>[5x]MNEAVKTLDGWFCLHDFRSIDWAAWRELNPGNQELMLNELSHFLSDMEITKNIGEGEHTIYSILGQKADLVFFTLRDSLEALNEVENRFNKLAIADYLLPTYSYISVVELSNYLASHMAGGDDPYQNKGVRARLYPALPPKKHICFYPMSKKRDG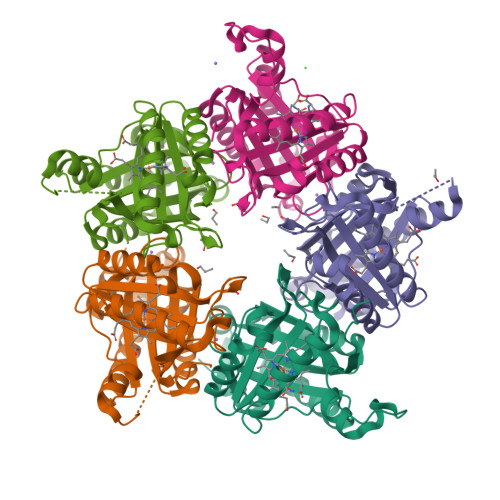ADNWYMLPMEERQQLIRDHGLIGRSYAGKVQQIIGGSIGFDDYEWGVTLFSDDALEFKRIVTEMRFDEASARYAEFGSFFIGNLLLSEQLSKLFTI> EEKEMKPACIKALTRIFKISDQDNDGTLNDAELNFFQRICFNTPLAPQALEDVKNVVRKHISDGVADSGLTLKGFLFLHTLFIQRGRHETTWTVLRRFGYDDDLDLTPEYLFPLLKIPPDCTTELNHHAYLFLQSTFDKHDLDRDCALSPDELKDLFKVFPYIPWGPDVNNTVCTNERGWIT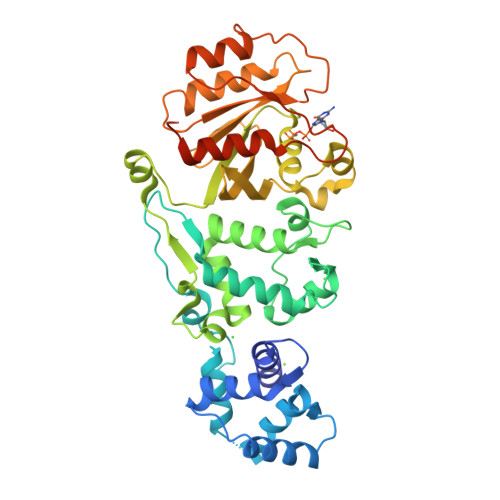YQGFLSQWTLTTYLDVQRCLEYLGYLGYSILTEQESQASAVTVTRDKKIDLQKKQTQRNVFRCNVIGVKNCGKSGVLQALLGRNLMRQKKIREDHKSYYAINTVYVYGQEKYLLLHDISESEFLTEAEIICDVVCLVYDVSNPKSFEYCARIFKQHFMDSRIPCLIVAAKSDLHEVKQEYSISPTDFCRKHKMPPPQAFTCNTADAPSKDIFVKLTTMAMYPHVTQADLKSSTFLEHHHHHH> MNHKVHHHHHHNLQTFELPTEVTGCAADISLGRALIQAWQKDGIFQIKTDSEQDRKTQEAMAASKQFCKEPLTFKSSCVSDLTYSGYVASGEEVTAGKPDFPEIFTVCKDLSVGDQRVKAGWPCHGPVPWPNNTYQKSMKTFMEELGLAGERLLKLTALGFELPINTFTDLTRDGWHHMRVLRFPPQTSTLSRGIGAHTDYGLLVIAAQDDVGGLYIRPPVEGEKRNRNWLPGESSAGMFEHDEPWTFVTPTPGVWTVFPGDILQFMTGGQLLSTPHKVKLNTRERFACAYFHEPNFEASAYPLFEPSANERIHYGEHFTNMFMRCYPDRITTQRINKENRLAHLEDLKKYSDT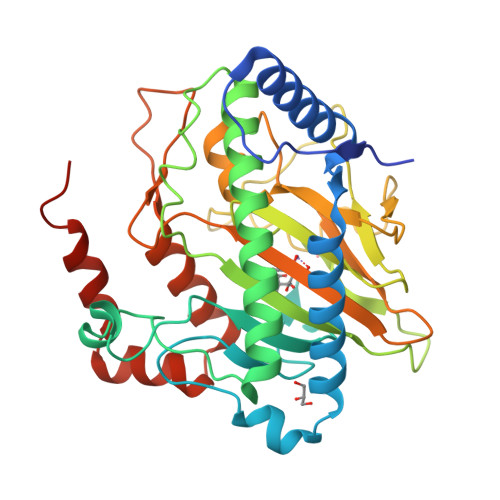RATGS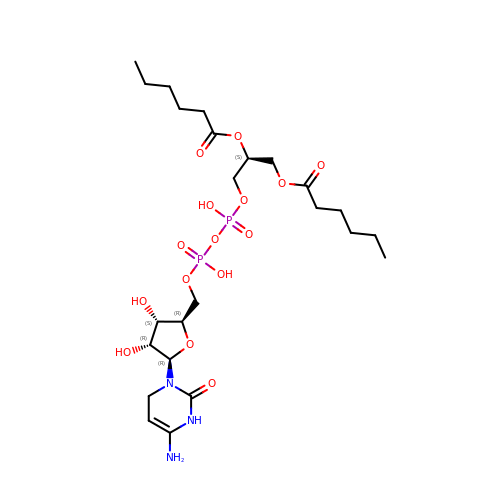[(2~{S})-3-[[[(2~{R},3~{S},4~{R},5~{R})-5-(6-azanyl-2-oxidanylidene-1,4-dihydropyrimidin-3-yl)-3,4-bis(oxidanyl)oxolan-2-yl]methoxy-oxidanyl-phosphoryl]oxy-oxidanyl-phosphoryl]oxy-2-hexanoyloxy-propyl] hexanoate | C24 H43 N3 O15 P2 | ZCBKOYRYPJUKTK-PFMQYRJWSA-N>AYKLVCYFTNWSQDRQEPGKFTPENIDPFLCSHLIYSFASIENNKVIIKDKSEVMLYQTINSLKTKNPKLKILLSIGGYLFGSKGFHPMVDSSTSRLEFINSIILFLRNHNFDGLDVSWIYPDQKENTHFTVLIHELAEAFQKDFTKSTKERLLLTAGVSAGRQMIDNSYQVEKLAKDLDFINLLSFDFHGSWEKPLITGHNSPLSKGWQDRGPSSYYNVEYAVGYWIHKGMPSEKVVMGIPTYGHSFTLASAETTVGAPASGPGAAGP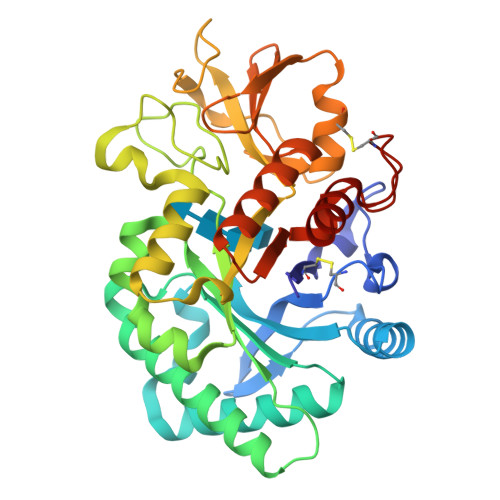ITESSGFLAYYEICQFLKGAKITRLQDQQVPYAVKGNQWVGYDDVKSMETKVQFLKNLNLGGAMIWSIDMDDFTGKSCNQGPYPLVQAVKRSLGSL[12x]> DNCDPENGKKVYQICSVCHSNDTTGVHGAAAPNLHGLEGRKVGSVPGFKFSSALRDSGDTWTPQHLD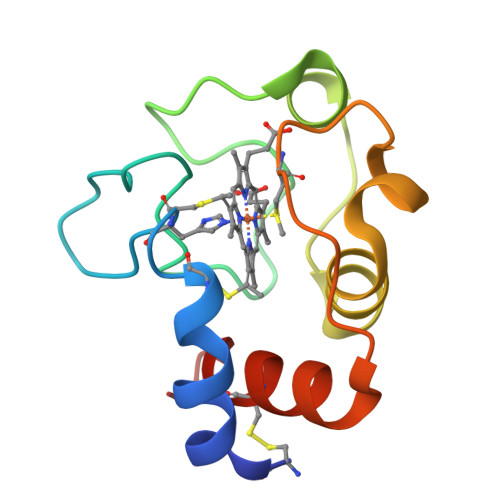KFLENPMAVYPLTRMAFSGLKNEKDRRDVLCFLSKSSN> MSFESKKPMRTWSHLAEMRKKPSEYDIVSRKLHYSTNNPDSPWELSPDSPMNLWYK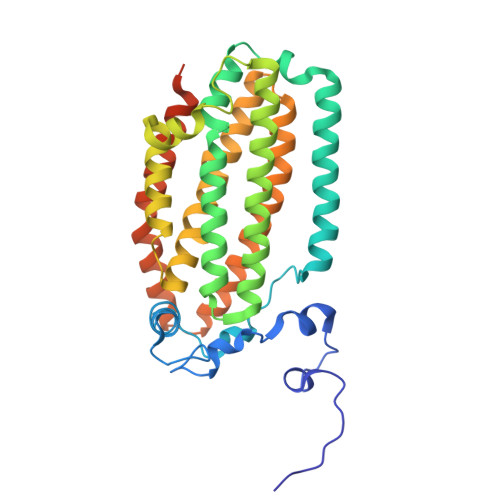QYRNASPLKHDNWDAFTDPDQLVYRTYNLMQDGQESYVQSLFDQFNEREHDQMVREGWEHTMARCYSPLRYLFHCLQMSSAYVQQMAPASTISNCCILQTADSLRWLTHTAYRTHELSLTYPDAGLGEHERELWEKEPGWQGLRELMEKQLTAFDWGEAFVSLNLVVKPMIVESIFKPLQQQAWENNDTLLPLLIDSQLKDAERHSRWSKALVKHALENPDNHAVIEGWIEKWRPLADRAAEAYLSMLSSDILHAQYLERSTSLRASILTV> TRCTHLENRDFVTGVQGTTRVSLVLELGGCVTITAEGKPSIDVWLEDIFQESPAETREYCLHAKLSNTKVEARCPTTGPATLPEEHQANMVCKRDQSDRGWGNHCGFFGKGSIVACAKFECEEAKKAVGHVYDSTKITYVVKVEPHTGDYQAANETNENRKTAQFTVASEKVILDLGDYGDVSLTCKVASGIDVAQTVVMSLGSSKDHLPSAWQLHRDWFEDLALPWKHKDNQDWNSVEKLVEFGPPHAVKMDIFNLGDQTAVLLKSLAGVPLASVDN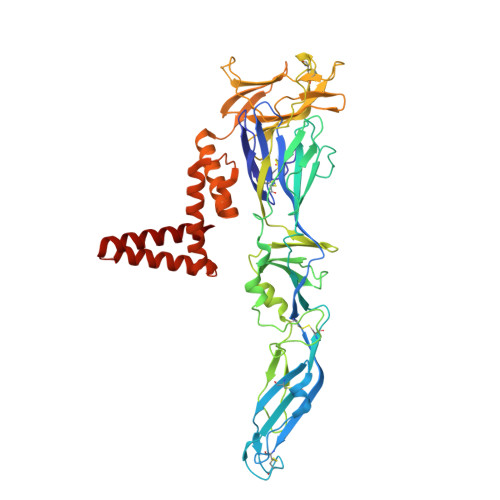QKYHLKSGHVTCDVGLEKLKLKGTTYSMCDKTKFKWKRVPVDSGHDTVVMEVSYTGSDKPCRIPVRAVAHGVPTINVAMLITPNPTIETSGGGFIEMQLPPGDNIIYVGDLSQQWFQKGSTIGRMFEKTRKGLERLSVVGEHAWDFGSVGGILSSVGKAIHTVLGGAFNTLFGGVGFIPKMLLGVALVWLGLNARNPTMSMTFLAVGALTLMMTMG>[2x]AGGGYWHTSGREILDANNVPVRIAGINWFGFETCNYVVHGLWSRDYRSMLDQIKS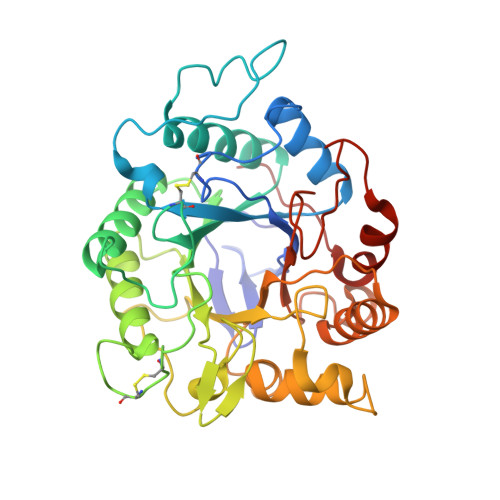LGYNTIRLPYSDDILKPGTMPNSINFYQMNQDLQGLTSLQVMDKIVAYAGQIGLRIILDRHRPDCSGQSALWYTSSVSEATWISDLQALAQRYKGNPTVVGFDLHNEPHDPACWGCGDPSIDWRLAAERAGNAVLSVNPNLLIFVEGVQSYNGDSYWWGGNLQGAGQYPVVLNVPNRLVYSAHDYATSVGPQTWFSDPTFPNNMPGIWNKNWGYLFNQNIAPVWLGEFGTTLQSTTDQTWLKTLVQYLRPTAQYGADSFQWTFWSWNPDSGDTGGILKDDWQTVDTDKDGYLAPIKSSIFDPV> MHHHHHHGSGMALAIKKRVGTYVETVDGSPPVKKLRLQTLAADAKGGKSGKVGNVERKLTALNQLDAYVGNLPAGALVLPTGTPVASTGAPSTGVIGNPPAAATGAPPMTAANSRELLELLVKITDEISYEDVEMGELKEVASKIFQLYQLQERDSDTSIRVKLLELLSGLGCECATEQALTMIIDY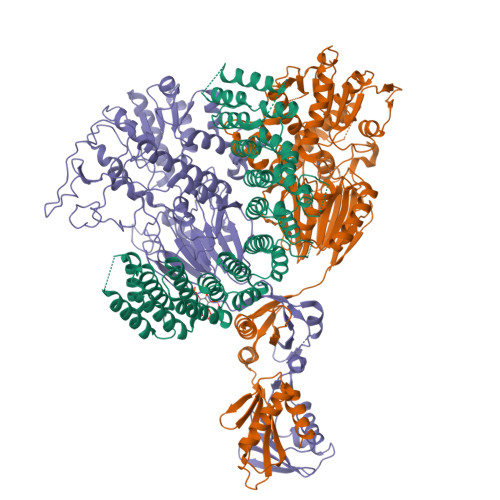FIFLLRKEVSQKVLAQGMMCLFRIGERRKHMLPISYKTQVAHLAKEQLRSGSAHTQKNAMLVIGRFATKMEGERHYVWKLAFYIDSQDSSVRAQALHALLTLGERGSQLPAVLYKRAVEAMKDDYECVRKEALQLVFMLGNRHPDYILPSDRQQEELRMIDAAFSKVCEALCDLSLQIRVLAAELLGGMTAVSREFLHQTLDKKLMSNLRRKRTAHERGARLVASGEWSSGKRWADDAPQEHLDAQSISIIASGACGALIHGLEDEFLEVRTAAVASMCKLALSRPDFAVTSLDFLVDMFNDEIEDVRLKAIYSLTAIAKHIVLREDQLEIMLGSLEDYSVDVREGLHLMLGACRVSTQTCLLMVVQKLLDVLAKYPQDRNSTYACMRKIGQKHPHLVMAVAVHLLYVHPFFETPERDVEDPAYLCVLILVFNAAEHLVPIISLLPTATHRHYAYLRDSMPNLVPQLPIEGASSASATHRIDSAMHQAGSSAEYLQMILSHIEEIFTMTDERLELLQTAQSNLQRLGSIDAGMYGTSNFLETFLAAQIQIEQMQRCASTQRSRVPLKESLAALIRNCLKLQHTFSGLNYGDILQVKQLRLRACALHLVLVVRDRSQSALGPCQMLLQTAGDISEFIKANTKDEEEKPPVVETDMPMKESVSRDAQPDSFTRQLLIKLDGISDPKPGRVFREILPLVQQAPPLALPPANDKIRRCVANILEPCPLQSQDNVIKVTAGLIAAVPFVAEIDNLLESQKADMRIKIKYPDQHMHTVVPKQSDFKPIMTEQGEHKTNVRLRTTILLSHSVWTESSLVEIQLCLAVRPGSELELCKPAKVLFAPKPVRRGI;> MRLYCLSGDLAKPCYIITFKGLRIMLDCGLTEQTVLNFLPLPFVQSLKWSNLPNFVPSRDHDPQMDGELKDCCGRVFVDSTPEFNLPMDKMLDFSEVDVILISNYLNMLALPYITENTGFKGKVYATEPTLQIGRFFLEELVDYIEVSPKACTARLWKEKLHLLPSPLSEAFRAKKWRTIFSLKDVQGSLSKVTIMGYDEKLDILGAFIATPVSSGYCLGSSNWVLSTAHEKICYVSGSSTLTTHPRPINQSALKHADVLIMTGLTQAPTVNPDTKLGELCMNVALTIRNNGSALIPCYPSGVVYDLFECLTQNLENAGLNNVPMFFISPVADSSLAYSNILAEWLSSAKQNKVYLPDDPFPHAFYLRNNKLKHYNHVFSEGFSKDFRQPCVVFCGHPSLRFGDAVHFIEMWGNNPNNSIIFTEPDFPYLQVLAPFQPLAMKAFYCPIDTSLNYQQANKLIKELKPNVLVIPEAYTKPHPSAPNLFIEQPDKKIITFKCGEIIRLPLKRKLDRIYITSELAQKISPKEVAAGVTFSTLTGVLQVKDKVHCIQPCADSVKDETISSNSAPTKEDVLKNVKYEYGSIDVDAVMKKLAQDGFSNIKLDRTGGALTLNLVNEDTVIKFEDNETHIICGGKPTTRLKLRDTIMKCLQSF;> MPDIKITPLGAGQDVGRSCLLLSMGGKNIMLDCGMHMGYNDERRFPDFSYIVPEGPITSHIDCVIISHFHLDHCGALPYMSEIVGYTGPIYMTHPTKAIAPILLEDMRKVAVERKGESNFFTTQMIKDCMKKVIPVTLHQSMMVDTDLEIKAYYAGHVLGAAMFWIKVGSQSVVYTGDYNMTPDRHLGAAWIDKCRPDLLISESTYATTIRDSKRCRERDFLKKVHECVAKGGKVLIPVFALGRAQELCILLETYWERMNLKYPIYFALGLTEKANTYYKMFITWTNQKIRKTFVHRNMFDFKHIKPFDKAYIDNPGAMVVFATPGMLHAGLSLQIFKKWAPNENNMVIMPGYCVQGTVGNKILGGAKKVEFENRQVVEVKMAVEYMSFSAHADAKGIMQLIQNCEPKNVMLVHGEAGKMKFLRSKIKDEFNLETYMPANGETCVISTPVKIPVDASVSLLKAEARSYNAQPPDPKRRRLIHGVLVMKDNRIMLQNLTDALKEIGINRHVMRFTSKVKMDDSGPVIRTSERLKTLLEEKLAGWTVTMQENGSIAIESVEVKVEEDEKDPKQKNILISWTNQDEDIGAYILNVLQNMC>[13x]MAEKRTGLAEDGAKSVYERLKNDRAPYETRAQNCAQYTIPSLFPKDSDNASTDYQTPWQAVGARGLNNLASKLMLALFPMQTWMRLTISEYEAKQLLSDPDGLAKVDEGLSMVERIIMNYIESNSYRVTLFEALKQLVVAGNVLLYLPEPEGSNYNPMKLYRLSSYVVQRDAFGNVLQMVTRDQIAFGALPEDIRKAVEGQGGEKKADETIDVYTHIYLDEDSGEYLRYEEVEGMEVQGSDGTYPKEACPYIPIRMVRLDGESYGRSYIEEYLGDLRSLENLQEAIVKMSMISSKVIGLVNPAGITQPRRLTKAQTGDFVTGRPEDISFLQLEKQADFTVAKAVSDAIEARLSFAFMLNSAVQRTGERVTAEEIRYVASELEDTLGGVYSILSQELQLPLVRVLLKQLQATQQIPELPKEAVEPTISTGLEAIGRGQDLDKLERCVTAWAALAPMRDDPDINLAMIKLRIANAIGIDTSGILLTEEQKQQKMAQQSMQMGMDNGAAALAQGMAAQATASPEAMAAAADSVGLQPGI

The bacteriophage portal protein (also named connector) is found at a unique vertex of the viral capsid and is essential for procapsid assembly, genome encapsidation, tail assembly and genome ejection. Its overall architecture corresponds to a ring-like hollow cylindrical dodecamer. However, portals have also been described to be able to assemble as undecameric or tridecameric complexes after overexpression, although they are only incorporated into the procapsids as dodecamers. The portal protein of the T7 bacteriophage is coded by the gp8 gene and has a predicted molecular weight of 59 kDa, which would give a multimeric complex of 650–770 kDa, depending on its oligomerization state.

Nevertheless, self-rotation function (SRF) calculations performed with MOLREP indicated that the T7 portal was composed of 13 protomers in the data set 1 crystal. Comparing the peaks at χ = 30°, χ = 27.7° and χ = 25.7°, which would correspond to the presence of dodecameric, tridecameric or tetradecameric NCS, respectively, the highest peak was found to be in the χ = 27.7° section. Therefore, the complex present in the crystal was a tri­decamer, with one ring per asymmetric unit and with a solvent content of 49%. Eventually, the 3D classification of a subset of 1200 particles with RELION yielded a map of a tridecameric portal at 7.8 Å resolution. Built as polyalanine chains, the model consisted of nine α-helices. It contained 194 residues of the total of 536 amino acids present in the gp8 monomer. The resulting tridecameric partial model was used for MR with Phaser against data set 1. The model was then subjected to rigid-body refinement by protomer using REFMAC5, which moved all of the protomers significantly (3.5 Å) towards the central channel, shrinking the particle diameter and central channel. Solvent flattening, histogram matching and NCS averaging were applied with masks generated from the cryo-EM map. The correlation between NCS-related regions of the map was 0.849. This DM procedure yielded a fully interpretable electron-density map of the particle.MJ0927 is a member of the Nif3 family and is highly conserved among bacteria and humans. The crystal structure of MJ0927 determined at 2.47 Å revealed that MJ0927 folds into two interlinked α/β domains. Six protomers of MJ0927 are found to form a novel hollow cage-like hexamer, in contrast to the toroid-shaped hexamers formed by other members of the Nif3 family. Additionally, we found that MJ0927 is a DNA-binding protein exhibiting the ability to bind to both single-stranded DNA (ssDNA) and double-stranded DNA (dsDNA).

Two crystal forms of MJ0927 were obtained, one in the P21 and the other in the C2221 space groups. The refined structure was subsequently used as the template to solve the native C2221 structure by a molecular replacement approach. The C2221 crystal form contains a single copy of a trimer in each asymmetric unit. No significant structural differences of the individual molecules were observed between the P21 and C2221 crystal forms. Since MJ0927 is a thermophilic archaeal Nif3 protein, it is not surprising that the quaternary structure of MJ0927 differs from other bacterial Nif3 proteins with regard to the stabilizing structural elements, particularly the structural arrangement at the intratrimer interfaces. As seen in Figure 2(b), the intratrimer interfaces are tightly packed between the second domains of MJ0927 and the three subunits are arranged in a tail-to-tail manner. The surface area of each subunit buried in the intratrimer interface is 1110 Å2, representing ~9.1% of the surface area of each subunit. There are five direct hydrogen bonds and six salt bridges and extensive hydrophobic interactions between the monomers across the intratrimer interface. Therefore, the trimer organization of MJ0927 is a unique structural feature that likely contributes to its increased structural stability and which has never been observed in other Nif3 proteins. However, no metal ion was observed in the metal-binding site of MJ0927 even though MJ0927 contains these conserved residues.

>[3x]MKAKEIIEFIETFAPKDLAIEGDNIGLQVGDNLDKEIKKLGIALDPSLSVIKKAEKEGVDFLFTHHPLLKDPIRNFTGVIYKKLKILMENDIILYSAHTNLDICKNGLNDALAELYNLENPKPLYDNGLGRVGIFKGSFEEFLEITKKYIHKNPIVVKSKEVDDNFKLAVLSGYGLSQSSIKYVAEKADVYLSGDLTHHSKILAEELGLVVVDATHYSTEVFGLKKFKEFLSSNLDLEIISLDFLEHHHHHH> MKEFYISIETVGNNIVERYIDENGKERTREVEYLPTMFRHCKEESKYKDIYGKNCAPQKFPSMKDARDWMKRMEDIGLEALGMNDFKLAYISDTYGSEIVYDRKFVRVANCDIEVTGDKFPDPMKAEYEIDAITHYDSIDDRFYVFDLLNSMYGSVSKWDAKLAAKLDCEGGDEVPQEILDRVIYMPFDNERDMLMEYINLWEQKRPAIFTGWNIEGFAVPYIMNRVKMILGERSMKRFSPIGRVKSKLIQNMYGSKEIYSIDGVSILDYLDLYKKFAFTNLPSFSLESVAQHETKKGKLPYDGPINKLRETNHQRYISYNIIDVESVQAIDKIRGFIDLVLSMSYYAKMPFSGVMSPIKTWDAIIFNSLKGEHKVIPQQGSHVKQSFPGAFVFEPKPIARRYIMSFDLTSLYPSIIRQVNISPETIRGQFKVHPIHEYIAGTAPKPSDEYSCSPNGWMYDKHQEGIIPKEIAKVFFQRKDWKKKMFAEEMNAEAIKKIIMKGAGSCSTKPEVERYVKFSDDFLNELSNYTESVLNSLIEECEKAATLANTNQLNRKILINSLYGALGNIHFRYYDLRNATAITIFGQVGIQWIARKINEYLNKVCGTNDEDFIAAGDTDSVYVCVDKVIEKVGLDRFKEQNDLVEFMNQFGKKKMEPMID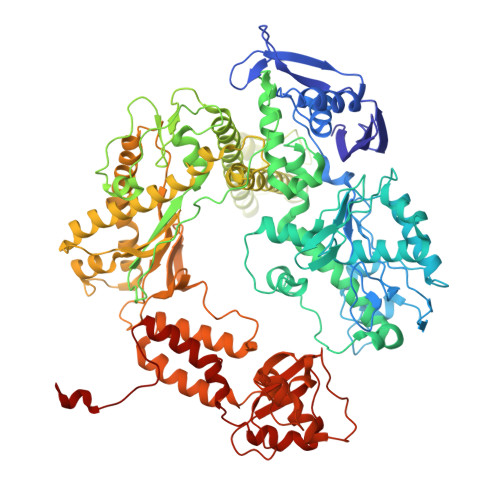VAYRELCDYMNNREHLMHMDREAISCPPLGSKGVGGFWKAKKRYALNVYDMEDKRFAEPHLKIMGMETQQSSTPKAVQEALEESIRRILQEGEESVQEYYKNFEKEYRQLDYKVIAEVKTANDIAKYDDKGWPGFKCPFHIRGVLTYRRAVSGLGVAPILDGNKVMVLPLREGNPFGDKCIAWPSGTELPKEIRSDVLSWIDHSTLFQKSFVKPLAGMCESAGMDYEEKASLDFLFG2,6-DICHLORO-4-(6-PIPERAZIN-1-YLPYRIDIN-3-YL)-N-(1,3,5-TRIMETHYL-1H-PYRAZOL-4-YL)BENZENESULFONAMIDE 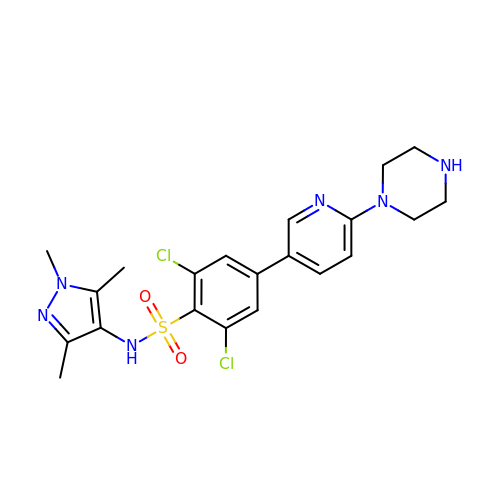| C21 H24 Cl2 N6 O2 S | HOIAFTVGAXSASA-UHFFFAOYSA-N>[2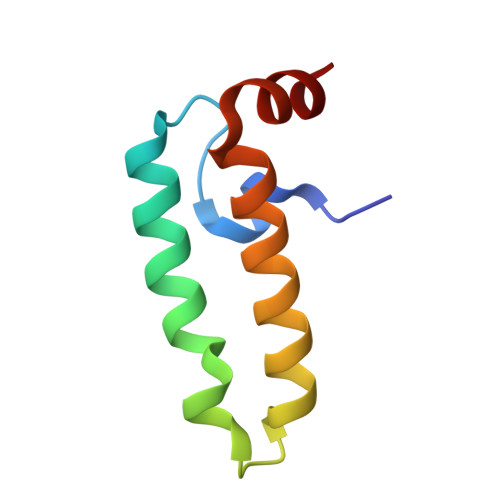x]GPMDYYTLLGVDKGCSEDDLRRAYLKLAMKWHPDKHVNKGSKVEAEEKFKNICEAYSVLSDNEKRVKYDL> GGCUUAUCAAGAGAGGGCGAGCGACUGGCGCGAAGAUCCCCGGCAACCAGAAAUGGUGCCAAUUCCUGCAGCGGAAACGUUGAAAGAUGAGCCG

One especially common junction element is the kink-turn (k-turn). k-turns are elements in double-stranded RNA that introduce a tight kink into the helical axis, with an included angle close to 50°. A standard k-turn comprises a three-nucleotide bulge followed by successive G•A and A•G trans G(sugar edge)•A(Hoogsteen edge) basepairs. k-turns are commonly-occurring motifs that introduce sharp kinks into duplex RNA, thereby facilitating tertiary contacts. Both the folding and conformation of k-turns are determined by their local sequence. k-turns fall into two conformational classes, called N3 and N1, that differ in the pattern of hydrogen bonding in the core. We show here that this is determined by the basepair adjacent to the critical G•A pairs.

We therefore decided to extend the study with a systematic structural analysis of HmKt-7 as a function of the 3b,3n sequence. This was performed in the constant environment of the SAM-I riboswitch, modified by replacing its natural k-turn by HmKt-7 with different 3b,3n sequences. In this way we could observe the effect of changing the 3b,3n sequence alone in an otherwise completely unchanged RNA molecule. Additionally, we hoped we might expand the range of 3b,3n sequences beyond the eight found in the natural k-turns to date. Six are completely new, i.e. 3b,3n = C•A, C–G, C•U, G•G, U–A and U•C, five of which adopt the N1 conformation. We note the majority (6/8) of the 3b = pyrimidine k-turns form N1 structures. Altogether seven of the new structures are in the N1 conformation, and clearly simply changing the 3b,3n sequence alone is sufficient to induce the structure of Kt-7 to change within the riboswitch environment. Evidently the 3b,3n sequence is the major determinant of the k-turn conformation.> MAAPGAGPGPGAPPGLEAALQKLALRRKKVLSAEETELFELAQAAGGAMDPEVFKILVDLLK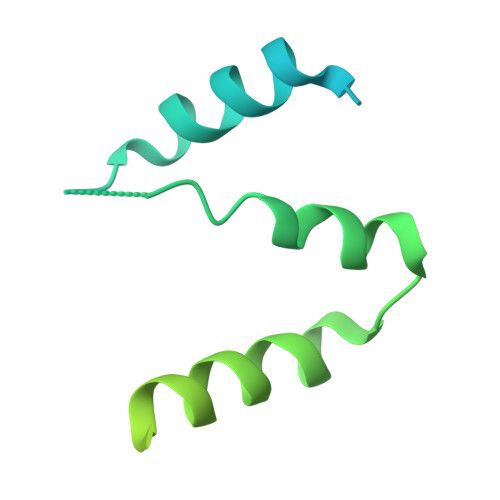LNVAPLAVFQMLKSMCAGQRLASEPQDPVAVPLPTTSVPETRGRNRGSSALGGGPALAERSGREGSSQRMPRQPSATRLPKGGGPGKSPTRST(5Z)-5-(3,5-difluoro-4-hydroxybenzylidene)-2-methyl-3-(2,2,2-trifluoroethyl)-3,5-dihydro-4H-imidazol-4-one 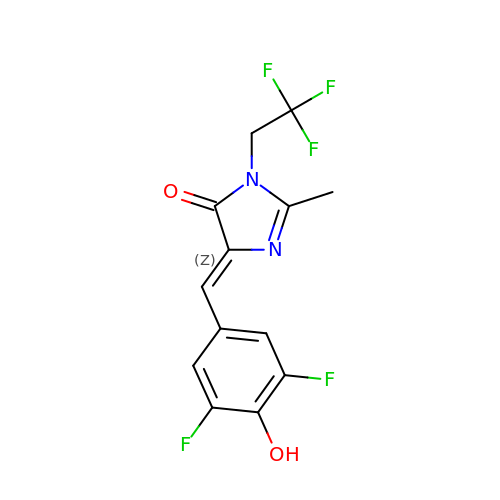| C13 H9 F5 N2 O2 | AWYCLBWNRONMQC-WMZJFQQLSA-N> MSNKERFLTLYHQIKSDANGYFSPEGIPYHSIETLICEAPDYGHMTTSEAYSYWLWLEVLYGHYTRDWSKLEAAWDNMEKYIIPVNEDGNDEQPHMSAYNPSSPATYASEKPYPDQYPSQLSGARPAGQDPIDGELKSTYGTNETYLMHWLLDVDNWYKYGNLLNPSHKAAYVNTFQRGQQESVWEAIPHPSQDDKSFGKPNEGFMSLFTKENQVPAAQWRYTNATDADARAIQAIYWAKELGYNNSTYLDKAKKMGDFLRYGMYDKYFQTIGSGKQGNPYPGNGKGACHYLMAWYTSWGGGLGDYANWSWRIGASHCHQGYQNPVAAYALSSDKGGLKPSSATGASDWEKTLKRQLEFYVWLQSKEGAIAGGATNSWNGDYSAYPAGRSTFYDMAYEDAPVYHDPPSNNWFGMQAWPMERVAELYYIFVKDGDKTSENVQMAKSCITKWVNYALDYIFIGSRPVSDEEGYFLDDQGRRILGGTNATVATTSAPGEFWLPGNIAWSGQPDTWNGFQSATGNPNLTAVTKDPTQDTGVLGSLVKAFTFFAAATKLETGNYTALGVRAKDAAAQLLEVAWNYNDGVGIVTEEEREDYDRFFKKEVYFPNGWNGTFGQGNQIPGSSTIPSDPQRGGNGVYTSFADLRPNIKQDPAWSSLESKYQSSFNEATGKWENGAPVFTYHRFWSQVDMATAYAEYHRLINLEHHHHHH

Enzymes in the glycoside hydrolase family 48 are believed to be an important member of many bacterial cellulase systems which also lack the better studied GH6 and GH7 family cellobiohydrolases produced by most cellulolytic fungi. All GH48 domains have (α/α)6 barrel fold with nearly identical organization of the active site tunnel. Out of 36 residues that represent the tunnel walls and contact with the substrate/product, 27 are universally conserved and most of the rest are highly conserved. To broaden the structural database and directly correlate activity to structural features, we have characterized and expressed two GH48 domains from C. bescii and B. pumilus and solved their structures using X-ray crystallography.

BpumGH48 Structure. a Cartoon representation of BpumGH48 structure with cellobiose and cellohexaose. α-helices are shown in red, β-strands in yellow and loops in green. The most unique feature about the structure of BpumGH48 is the eight unusually long peptide inserts that result in extra loops on the surface of the molecule when compared to other GH48 enzymes. Beyond these loops, the core structure is very similar to other well described GH48 enzymes, such as CelF GH48, CelS GH48, or T. fusca GH48. Loop 5 (Leu303 to Asn308) is located near the tunnel entrance and loops 2 (Arg463 to Ala493) and 6 (Phe664 to Gly674) are near the exit. Due to their position, these loops have the potential to affect substrate-binding and product expulsion. Although, computer simulations indicate that the BpumGH48 loops near the tunnel exit do not affect product inhibition. However, they could be one of the reasons for the lower thermostability of BpumGH48 by being more exposed to solvent. The melting temperatures for purified GH48 enzymes isolated from C. bescii, T. fusca, and B. pumilus, were determined to be 80, 65, and 45 °C, respectively. The B. pumilus GH48 seems to outperform the other two GH48 enzymes by a small margin all at their optimal operating temperatures. Out of these, CelF is most similar.> MGSSHHHHHHSSGRENLYFQGSSWKWVSTGPLVFPKNDERNIAGIKDPTAVLINGTYHVFASTAKSEGYNMVYFNFTDFAEANNAPFYYLDQAPLGYGYRAAPQVFYFEPHKLWYLVYQNGNAAYSTNPDINDPSKWTAPEVFYPNGMPKIIADNIGNGYWVDMWVVCDDEEDPNKALCHLFSSDDNGHLYRSQTTLAQFPRGMSEPEIVLQDTQNIYALWEAACIYRIKGAEGTQKYLLLVEAIGQEGHRYFRSWTSDRIDGQWIPLADTEANPWAGEANVVFEGQKWTKSISHGEVIRTLTDQTLTLDLSEPIQFLYQGVDP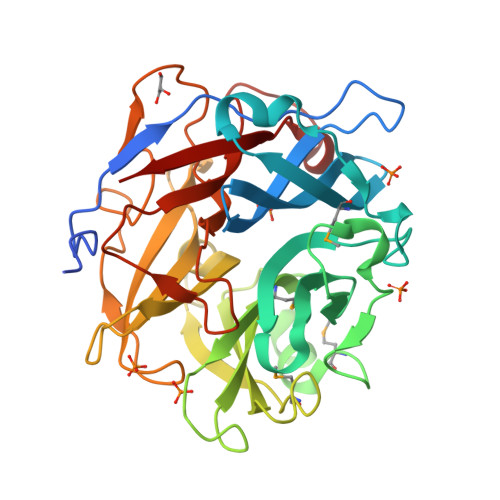NAQTEYNALPWRLGLITQ> GSHMGALKPAKAIVE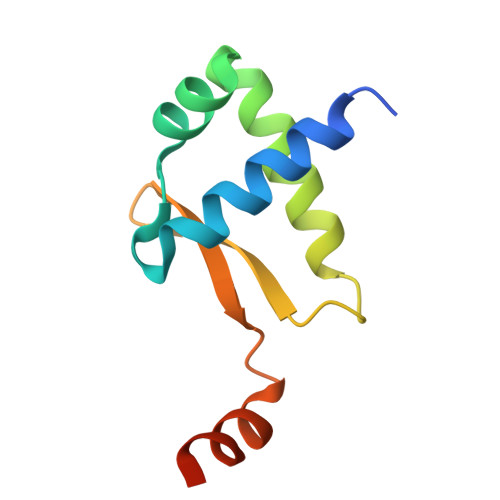ALLFAAGDEGLSLSQIAAVLEVSELEAKAVIEELQQDCRREERGIQLVELGGVFLLATKKEHAPYLKKLVEAPGASP Asparaginases (EC 3.5.1.1), which split L-asparagine to L-aspartate and ammonia, are grouped into three unrelated structural classes: Class 1 (bacterial-type), Class 2 (plant-type), and Class 3 (Rhizobium etli-type). ReAV is a homodimer with an α/β protomeric fold, formed by two tightly packed domains. The active site of the enzyme is located in a cleft on the protomer surface and marked by a zinc ion with an unusual coordination sphere created by Cys135, Lys138, Cys189, and a water molecule. The conspicuous catalytic center of the enzyme comprises two Ser-Lys tandems (Ser48-Lys51 and Ser80-Lys263), centered around the curiously hydrated Ser48 residue and located in the close vicinity of the metal binding site.

As in the structure with the C135A mutation, the absence of Cys189 triggered a collapse of the metal coordination site and the C189A mutant protein is unable to bind the Zn2+ cation, as also corroborated by microcalorimetric titration of this protein with zinc. The mutation induced slight atomic shifts and structural rearrangements in the active site area, but these changes are not strictly equivalent in the two subunits of the dimer. Alternative conformers of Cys135 were found in protein chain B, where the major rotamer with refined occupancy of 0.8 retained its typical conformation and points to the Nζ atom of Lys51, while the minor rotamer is rotated toward the Oγ atom of Ser133. The hydration pattern of Ser48 is similar as in the WT protein, with a water triad centered around the Ser48 hydroxyl group. However in subunit B, the Ser48 side chain exists in two conformational states, with the major rotamer, with refined occupancy of 0.7, directed toward the Ser80 hydroxyl group, and the lower-occupancy rotamer pointing to the carbonyl O atom of Leu264. The pattern of H-bonds at the two lysine residues, Lys51 and Lys263, is practically the same as in the WT protein. Only one conformer of Asp187 is visible in the electron density maps, but intriguingly, its side chain points to the main chain N atoms of Ala189, Asn190 and Leu191, and not toward the side chain of Arg47, as observed in the previously described C135A and H139A mutant structures. Apart from the interaction with Arg47, the sulfate ion forms H-bonds to the N atom of Gly188 and to four water molecules, two of which belong to the hydration sphere of Ser48. The position of the sulfate ion is slightly shifted compared to its position in the D187A mutant structure, where the sulfate ion is bound right next to the water from the metal coordination sphere. As in the case of the C135A and K138A variants lacking the metal cation, the mutation affected the oxidative state of Cys249, which is not oxidized.

>GIDPFTMTPSEDFVVTDRGGIVENSHRVHAAVVDAKGRLLYALGNPTRMTLARSAAKPAQALAILETEGVAGYGFDDADIALMCASHSSEDRHIARTRAMLSKIKAEEADLRCGGHPSLSEMVNRSWIKQDFIPTAVCSNCSGKHVGMLAGARAIGAGTDGYHLPDHPMQGRVKRTVAELCDLDAGDVEWGTDGANLPTPAFPLDRLGRIYAKLASAADGSDAGEGQSTRCAALAHIFRAMARHPEMVAGEGRYCTMLMRAFDGALVGKLGADASYAIGVRASDATRQLGTDGALGISVKIEDGNLEMLYAVVTELLERLGIGSPDVRSQLASFHHPQRVNTMGVTTGGVSFPFKLRGSKSNVDDPRLAAVAR[2x]>[2x]ASKPQPIAAANWKCNGSESLLVPLIETLNAATFDHDVQCVVA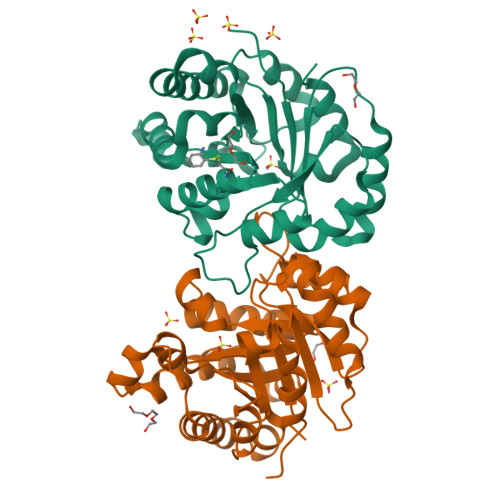PTFLHIPMTKARLTNPKFQIAAQNAITRSGAFTGEVSLQILKDYGISWVVLGHSERRLYYGETNEIVAEKVAQACAAGFHVIVCVGETNEEREAGRTAAVVLTQLAAVAQKLSKEAWSRVVIAYEPVWAIGTGKVATPQQAQEVHELLRRWVRSKLGTDIAAQLRILYGGSVTAKNARTLYQMRDINGFLVGGASLKPEFVEIIEATK>[2x]GSTGGVQTVTLIPGDGIGPEISAAVMKIFDAAKAPIQWEERNVTAIQGPGGKWMIPSEAKESMDKNKMGLKGPLKTPIAAGHPSMNLLLRKTFDLYANVRPCVSIEGYKTPYTDVNIVTIRENTEGEYSGIEHVIVDGVVQSIKLITEGASKRIAEFAFEYARNNHRSNVTAVHKANIMRMSDGLFLQKCREVAESCKDIKFNEMYLDTVCLNMVQDPSQFDVLVMPNLYGDILSDLCAGLIGGLGVTPSGNIGANGVAIFESVHGTAPDIAGKDMANPTALLLSAVMMLRHMGLFDHAARIEAACFATIKDGK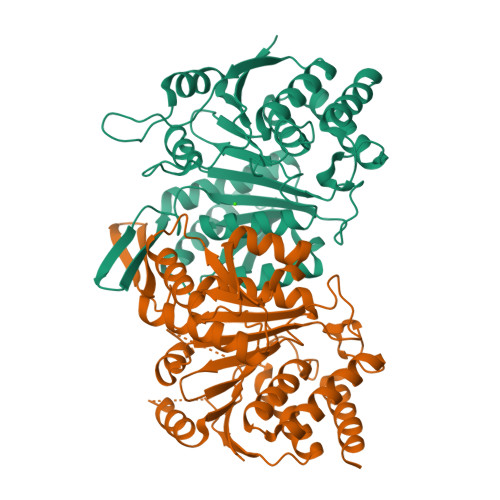SLTKDLGGNAKCSDFTEEICRRVKDLD;>[2x]ASRSQAEDVRVEGSFPVTMLPGDGVGPELMHAVKEVFKAAAVPVEFQEHHLSEVQNMASEEKLEQVLSSMKENKVAIIGKIHTPMEYKGELASYDMRLRRKLDLFANVVHVKSLPGYMTRHNNLDLVIIREQTEGEYSSLEHESARGVIECLKIVTRAKSQRIAKFAFDYATKKGRGKVTAVHKANIMKLGDGLFLQCCEEVAELYPKIKFETMIIDNCCMQLVQNPYQFDVLVMPNLYGNIIDNLAAGLVGGAGVVPGESYSAEYAVFETGARHPFAQAVGRNIANPTAMLLSASNMLRHLNLEYHSSMIADAVKKVIKVGKVRTSDMGGYATCHDFTEEICRRVKDLDENLYFQ> MGRLLALVVGAALVSSACGGCVEVDSETEAVYGMTFKILCISCKRRSETNAETFTEWTFRQKGTEEFVKILRYENEVLQLEEDERFEGRVVWNGSRGTKDLQDLSIFITNVTYNHSGDYECHVYRLLFFENYEHNTSVVKKIHIEVVDKAN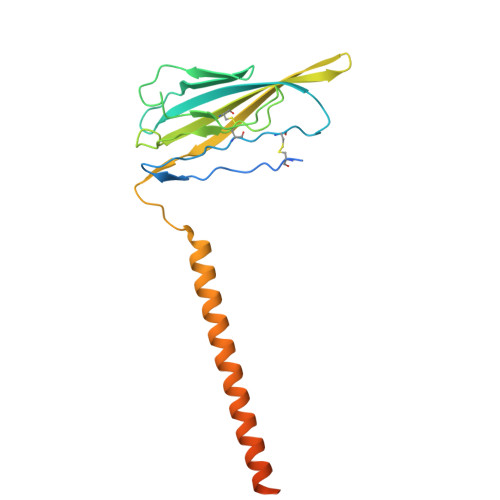RDMASIVSEIMMYVLIVVLTIWLVAEMIYCYKKIAAATETAAQENASEYLAITSESKENCTGVQVAE>[2x]SSRKAKKKA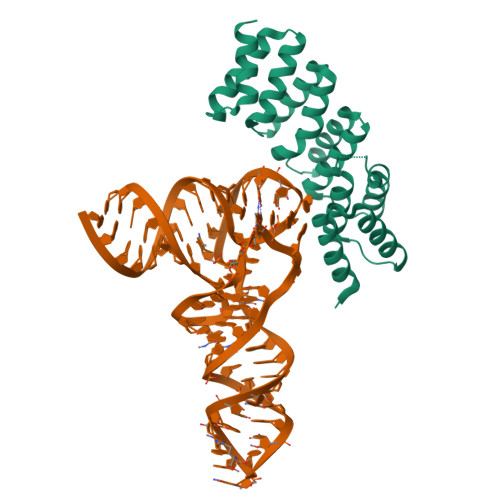IQQSPEALLKQKLDMCSKKGDVLEALRLYDEARRNGVQLSQYHYNVLLYVCSLASASSNPGLSRGFDIFKQMIVDKVVPNEATFTNGARLAVAKDDPEMAFDMVKQMKAFGIQPRLRSYGPALFGFCRKGDADKAYEVDAHMVESEVVPEEPELAALLKVSMDTKNADKVNKTLQRLRDLVRQVSKSTQDMIEEWQKSE>TGTPVERYGKVQVCGTQLCDEHGNPVQLRGMSTHGIQWFDHCLTDSSLDALAYDWKADIIRLSMYIQEDGYETNPRGFTDRMHQLIDMATARGLYVIVDWHILTPGDPHYNLDRAKTFFAEIAQRHASKTNVLYEIANEPNGVSWASIKSYAEEVIPVIRQRDPDSVIIVGTRGWSSLGVSEGSGPAEIAANPVNASNIMYAFHFYAASHRDNYLNALREASELFPVFVTQFGTETYTGDGANDFQMADRYIDLMAERKIGWTKWNYSDDF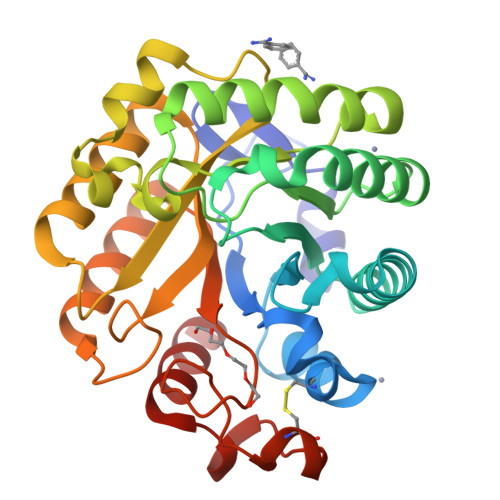RSGAVFQPGTCASGGPWSGSSLKASGQWVRSKLQS[2x]>GPSSPAHVIFQNVAKSYLPNAHLECHYTLTPYIHPHPKDWVGIFKVGWSTARDYYTFLWSPMP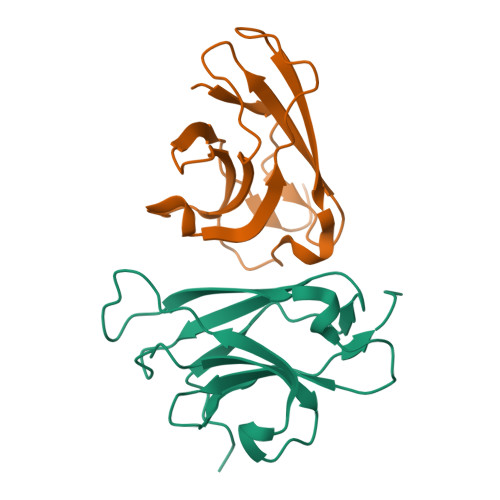EHYVEGSTVNCVLAFQGYYLPNDDGEFYQFCYVTHKGEIRGASTPFQFRASSPVEELLTMEDEGNSDMLVVTTKA[2x]> MTGGMKPPARKPRILNSDGSSNITRLGLEKRGWLDDHYHDLLTVSWPVFITLITGLYLVTNALFALAYLACGDVIENARPGSFTDAFFFSVQTMATIGYGKLIPIGPLANTLVTLEALCGMLGLAVAASLIYARFTRPTAGVLFSSRMVISDFEGKPTLMMRLANLRIEAIIEADVHLVLVRSEISQEGMVFRRFHDLTLTRSRSPIFSLSWTVMHPIDHHSPIYGETDETLRNSHSEFLVLFTGHHEAFAQNVHARHAYSCDEIIWGGHFVDVFTTLPDGRRALDLGKFHEIAQHHHHH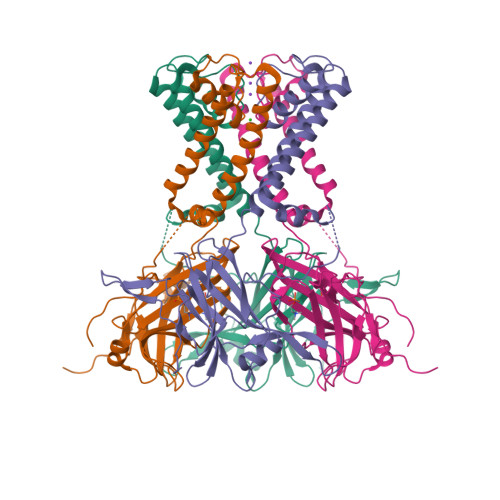H4-(diethylamino)benzohydrazide | 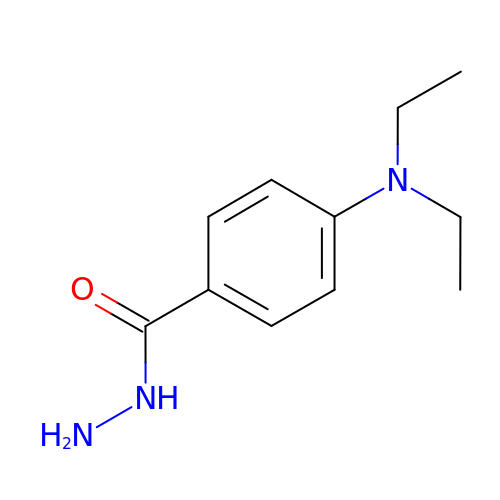C11 H17 N3 O | PUNSOBLTEWFAMJ-UHFFFAOYSA-N> PEEERIKYVITVVEQIAKDAHRNGQEELAKLAERTAEEAKKATERGEEETLRIVYVIVVVLQIALEAHRNGQEELAKLALRTAEEAIKATERGEEETLRIVYVIVVVLQIALEAHRNGQEELAKLALRTAEEAIKATERGEEETLRIVYVIVVVLQIALEAHRNGQEELAKLALRTAEEAIK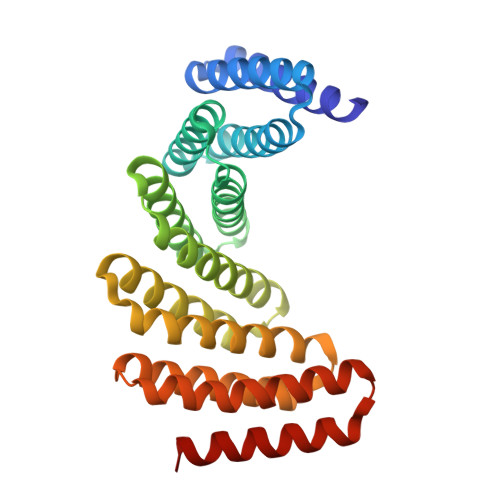ATERGEEETLRIVYVIVVVLQIALEAHRNGQEELAKLALRTAEEAIKATERGEEETERIVYDIVVVLQEALEAHRNGEEERAKKALDEARRRIEATERGE>GSHMSGIALSRLAQERRAWRKDHPFGFVAVPTKNPDGTMNLMNWECAIPGKKGTPWEGGLFKLRMLFKDDYPSSPPKCKFEPPLFHPNVYPSGTVCLSILEEDKDWRPAITIKQILLGIQELLNEPNIQDPAQAEAYTIYCQNRVEYEKRVRAQAKKFAPS[2x];>[2x]GSHMNDHINLKVAGQDGSVVQFKIKRHTPLSKLMKAYCERQGLSMRQIRFRFDGQPINETDTPAQLEMEDEDTIDVFQQQTGG;>[2x]SNTGEPAPVLSSPPPADVSTFLAFPSPEKLLRLGPKSSVLIAQQTDTSDPEKVVSAFLKVSSVFKDEATVRMAVQDAVDALMQKAFNSSSFNSNTFLTRLLVHMGLLKSEDKVKAIANLYGPLMALNHMVQQDYFPKALAPLLLAFVTKPNSALESCSFARHSLLQTLYKV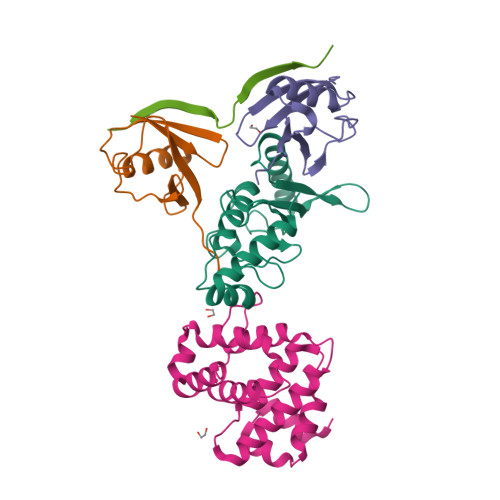;> GAMDHVEFGSGDPGSEIIESVPPAGPEASESTTDENEDDIQFVSEGPLRPVLEYIDLVSSDDEEP>MGSSHHHHHHSQDPMLSVGATTTATRLTGWGRTAPSVANVLRTPDAEMIVKAVARVAESGGGRGAIARGLGRSYGDNAQNGGGLVIDMTPLNTIHSIDADTKLVDIDAGVNLDQLMKAALPFGLWVPVLPGTRQVTVGGAIACDIHGKNHHSAGSFGNHVRSMDLLTADGEIRHLTPTGEDAELFWATVGGNGLTGIIMRATIEMTPTSTAYFIADGDVTASLDETIALHSDGSEARYTYSSAWFDAISAPPKLGRAAVSRGRLATVEQLPAKLRSEPLKFDAPQLLTLPDVFPNGLANKYTFGPIGELWYRKSGTYRGKVQNLTQFYHPLDMFGEWNRAYGPAGFLQYQFVIPTEAVDEFKKIIGVIQASGHYSFLNVFKLFGPRNQAPLSFPIPGWNICVDFPIKDGLGKFVSELDRRVLEFGGRLYTAKDSRTTAETFHAMYPRVDEWISVRRKVDPLRVFASDMARRLELL[2x]

DprE1 is the first of two enzymes that catalyze the conversion of decaprenylphosphoryl-β-D-ribose (DPR) to decaprenylphosphoryl-β-D-arabinose (DPA). In its natural context, DprE1 catalyzes the oxidation of the 2′ hydroxyl group of DPR to give the ketone decaprenylphosphoryl-2-keto-β-D-erythropentofuranose (DPX), with flavin adenine dinucleotide (FAD) acting as the oxidant in the reaction. After BTZs have entered the catalytic pocket of DprE1 containing the reduced form of the flavin cofactor (FADH2), which was generated by oxidation of the substrate, the nitro group of the BTZs is reduced to nitroso which can then form a covalent bond with a nearby cysteine residue (Cys387, Mtb enzyme numbering). We obtained co-crystal structures of Mtb-DprE1 with BTZ compounds 1, 2, 9, and 12 and BOZ compound 5.

Compound 2 is the four-electron reduced form of 7, also referred to as hydroxylamino-BTZ, and was synthesized as a potential noncovalent inhibitor control. However, it turned out to be a novel mechanism-based suicide substrate (see later). The progress curves for 2 were also time dependent, which was not expected given that this hydroxylamine compound is the two-electron reduced form of the nitroso derivative, 1. These data could be explained if 2 is an alternative substrate of Mtb-DprE1 that reduces Eox to generate an ERED:1 complex, followed by covalent bond formation with Cys387. We incubated 10 µM Mtb-DprE1 with 20 µM of the hydroxylamino-BTZ 2 in the absence of FPR and resazurin and monitored the intact mass of the enzyme by mass spectrometry. The intensity of both species decreases with increasing incubation time, and two new species appear with molecular weights of 51986 Da and 52162 Da, which are 340–343 Da higher than the two starting species, consistent with the formation of the corresponding semimercaptal covalent derivatives. This hypothesis was further confirmed by X-ray data (see below) that clearly indicate a covalent bond to Cys387. The orientation of covalently-bound 2 in the active site of DprE1 is similar to the nitro and nitroso congeners. Therefore, 2 is a true mechanism-based suicide substrate of Mtb-DprE1 because substrate (DPR or FPR) is not required for covalent modification of Cys387 to occur. Very remarkably, 2 was very potent in the enzyme assay, surpassing its nitro analogue, 7.>[15x]TTSSQKFIARNRAPRVQIEYDVELYGAEKKVQLPFVMGVMADLAGKPAEPQAAVADRKFLEIDVDNFDARLKAMKPRVAFNVPNVLTGEGNLSLDITFESMDDFSPAAVARKVDSLNKLLEARTQLANLLTY;>REAVETAVRTLAEHALEQTSLISNDAIKSIESIIAALDAKLTAQVNLIMHHADFQQLESAWRGLHYLVNNTETDEQLKIRVLNISKPELHKTLKKFKGTTWDQSPIFKKLYEEEYGQFGGEPYGCLVGDYYFDQSPPDVELLGEMAKISAAMHAPFISAASPTVMGMGSWQELSNPRDLTKIFTTPEYAGWRSLRESEDSRYIGLTMPRFLARLPYGAKTDPVEEFAFEEETDGADSSKYAWANSAYAMAVNINRSFKLYGWCSRIRGVESGGEVQGLPAHTFPTDDGGVDMKCPTEIAISDRREAELAKNGFMPLLHKKNTDFAAFIGAQSLQKPAEYDDPDATANANLAARLPYLFATCRFAHYLKCIVRDKIGSFKEKDEMQRWLQDWILNYVDGDPAHSTETTKAQHPLAAAEVVVEEVEGNPGYYNSKFFLRPHYQLEGLTVSLRLVSKLPSAKEA[15x]

The type VI secretion system (T6SS) is a contractile injection machine widely distributed among Gram-negative bacteria. Bacteria use the T6SS to directly deliver effectors into bacteria or eukaryotic cells (Cianfanelli et al., 2016). The T6SS sheath comprises two proteins, TssB (VipA/IglA) and TssC (VipB/IglB), which form tubular structures similar to the T4 phage gp18 sheath (Leiman et al., 2009, Lossi et al., 2013, Clemens et al., 2015, Kudryashev et al., 2015). Upon sheath contraction the T6SS fires Hcp/VgrG and bound toxins and is subsequently recycled by the AAA+ ATPase ClpV, which binds the contracted sheath to disassemble it (Kapitein et al., 2013, Kube et al., 2014).

Here, we report the atomic structure of the TssB1C1 sheath encoded by the H1-T6SS cluster from P. aeruginosa. The 3D structure of TssB1C1 was obtained at 3.3 Å resolution using helical reconstruction within RELION (He and Scheres, 2017). The final 3D model of the 13-fold symmetric TssB1C1 sheath has a helical rise and twist of 20.2 Å and 27.7°, respectively, and presents a right-handed six-start helical assembly composed of discrete densities corresponding to the heterodimers. Side and cut-away views of the reconstruction show the 13-mer sheath as being composed of non-planar discs, each comprising 6.5 heterodimers for every 360° turn of the sheath due to a 3.36 Å axial rise difference between units. Since 12- and 13-fold symmetries are present, and given that all known contractile systems have 12-fold symmetry, we assume the 13-fold symmetry of the TssB1C1 sheath is due to sample preparation. The TssB1C1 heterodimer within the helical assembly of the sheath forms an intricate packing arrangement that is organized in three domains (domains 1, 2, and 3). Two β strands of TssC1 (β11 and β12) are joined by two donor β strands, one from a neighboring TssC1 subunit (β13) within the same protofilament and the other from an adjacent TssB1 subunit (β1) in a different protofilament, but within the same disc, to form a β sheet interaction (handshake interaction) at the inner layer of the sheath (domain 1). Two α helices (residues D117–L133 of TssB1 and S66–M86 of TssC1) and a third α helix (residues E39–E54 of TssC1) form a tri-helical bundle (domain 3; Figure 2Biii). This third α helix is in an extended conformation in our TssB1C1 sheath, radiating away from its originating heterodimer and interacting with an adjacent heterodimer directly below that belongs to a different protofilament, but is positioned within the same stile of the helical assembly. Our structure reveals key features for T6SS sheaths such as the extended TssC1 N-terminal α helix that forms an inter-protofilament tri-helical bundle at the outer layer of the contracted sheath.>[2x]MYGGFLRRIRPKLKWDNQGSGSHHWGSKEEEIEKEFEEKKKIIEENLKEAEEEGEEEAAEKLKEALKKLEEAIKLHREGANPVEV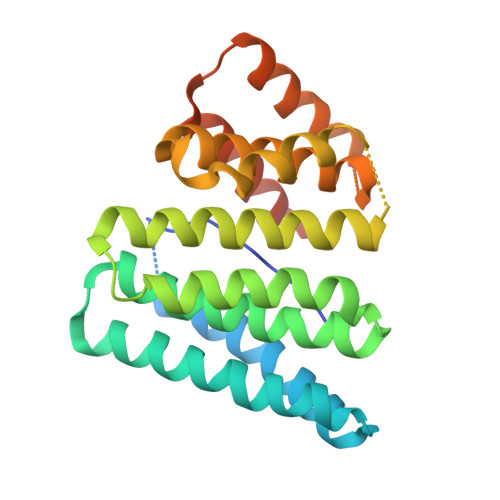ELEEVTAIILNNLAVLLREGEEELAKELEKAIKLLEEKKDAPEEERLKAIAIAIIRSVLVLIKWEGGKDEETIEEIEEILENRENLSLEELREAYVRAEIAYLIESGIDPEAAKKVREKYERGAPLEELLKDIEKIEKEAKKREEEKKLEHHHHHH>[2x]GSMAKIEKNAPTMEKKPELFNIMEVDGVPTLILSKEWWEKVCNFQAKPDDLILATYPKSGTTWMHEILDMILNDGDVEKCKRAQTLDRHAFLELKFPHKEKPDLEFVLEMSSPQLIKTHLPSHLIPPSIWKENCKIVYVARNPKDCLVSYYHFHRMASFMPDPQNLEEFYEKFMSGKVVGGSWFDHVKGWWAAKDMHRILYLFYEDIKKDPKREIEKILKFLEKDISEEILNKIIYHTSFDVMKQNPMTNYTTLPTSIMDHSISPFMRKGMPGDWKNYFTVAQNEEFDKDYQKKMAGSTLTFRTEI

Cytosolic sulfotransferases (SULTs) comprise a family of enzymes that catalyze the transfer of a sulfonate group from 3′-phosphoadenosine 5′-phosphosulfate (PAPS) to an acceptor group of the substrate. In doing so, SULTs modulate the activities of a large array of small endogenous and foreign chemicals, including drugs, toxic compounds, steroid hormones, and neurotransmitters. As expected, all SULTs share the same basic fold: a central four-stranded parallel β-sheet surrounded by α-helices and three loops that are often disordered (dashed lines) in the absence of PAP and/or substrate. The crystal structures of SULT1C3 bound to PAP, apo SULT1C2, a ternary complex of SULT1C2 bound to PAP, and the environmental toxin, pentachlorophenol (PCP), and SULT4A1 were solved at 3.2, 2.0, 1.8, and 2.2 Å, respectively.

Substrates for SULT1C3 have not been reported previously. Our data indicate that this recently identified member of the hSULT family is able to sulfonate p-nitrophenol, 1-naphthol, 2-ethylphenol, 2-n-propylphenol, and 2-sec-butylphenol, as well as the steroid-related compounds, α-zearalenol and lithocholic acid. SULT1C3 appeared to be most active with α-zearalenol (4.1 nmol/min/mg) and 2-ethylphenol (2.2 nmol/min/mg). These data suggest SULT1C3 may contribute to the metabolism of steroid and phenolic compounds. For example, both SULT1C3 and SULT1B1 were stabilized by catecholamines in the absence of PAP, but neither showed significant activity toward this class of compounds. We have identified a number of novel substrates, inhibitors, and compounds that bind to these SULTs in the absence of PAP. These data combined with activity assays revealed that SULT1C3 can bind catecholamines and phenolic compounds, but only the latter are substrates. However, a closer inspection of the structures also suggests that binding of substrates may not be completely uncoupled from binding of the cofactor. In all the structures with the co-factor product, PAP, α14-α15, and the C-terminal segment of the largest flexible loop (green in Figure 2) are ordered.>[3x]MAEREFDMTIEEVTIKVAPGLDYKVFGFNGQVPGPLIHVQEGDDVIVNVTNNTSLPHTIHWHGVHQKGTWRSDGVPGVTQQPIEAGDSYTYKFKADRIGTLWYHCHVNVNEHVGVRGMWGPLIVDPKQPLPIEKRVTKDVIMMMSTWESAVADKYGEGGTPMNVADYFSVNAKSFPLTQPLRVKKGDVVK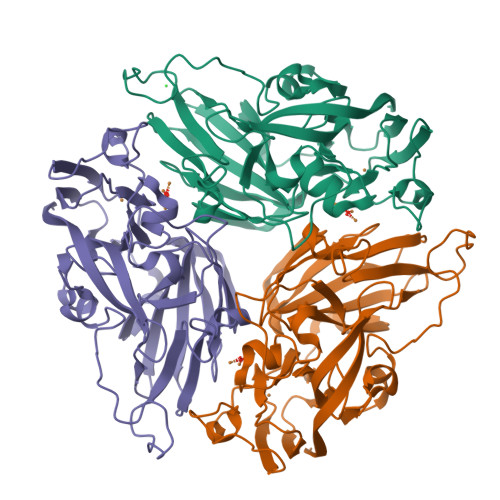IRFFGAGGGIHAMHSHGHDMLVTHKDGLPLDSPYYADTVLVSPGERYDVIIEADNPGRFIFHDHVDTHVTAGGKHPGGPITVIEYDGVPVDDWYVWKDKDYDPNFFYSESLKQGYGMFDHDGFKGEFEQRQRRPGRKLAAALEHHHHHH> KF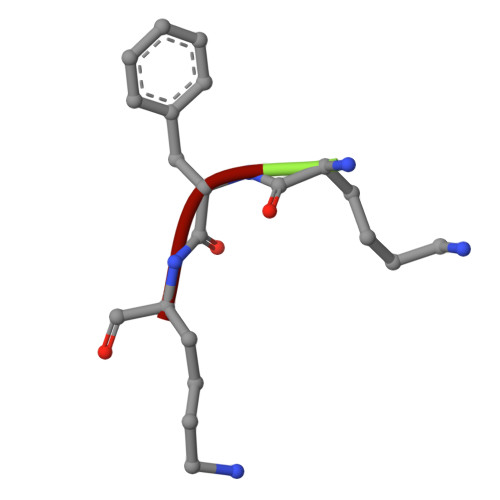K>[4x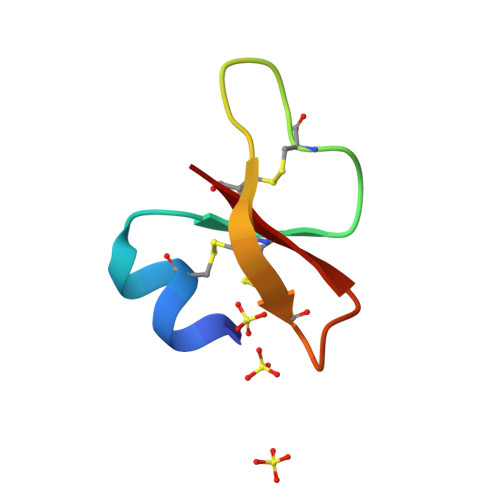]DHYNCVSSGGQCLYSACPIFTKIAGTCYRGKAKCCK> GHMASMAKIKNQYYNESVSPIEYAQQGFKGKMRSVNWNVVNDEKDLEVWNRITQNFWLPEKIPVSNDLTSWRTLTPEWQELITRTFTGLTLLDTIQATVGDVAQVPNSLTDHEQVIYTNFAFMVAVHARSYGSIFSTLCSSEQIEEAHEWVINTETLQERAKALIPYYVNDDP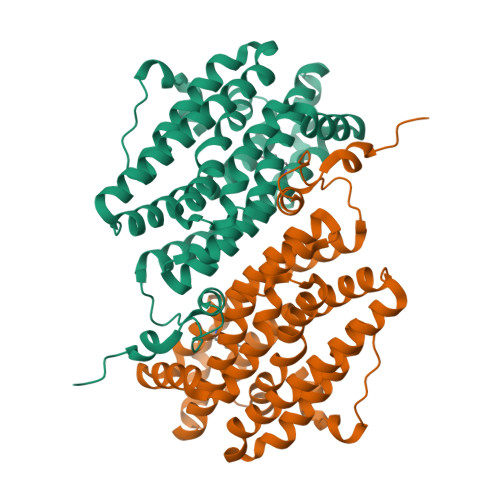LKSKVAAALMPGFLLYGGFYLPFYLSARGKLPNTSDIIRLILRDKVIHNYYSGYKYQKKVAKLSPEKQAEMKEFVFKLLYELIDLEKAYLKELYEDFGLADDAIRFSVYNAGKFLQNLGYDSPFTEEETRIEPEIFTQLSARADENHDFFSGNGSSYIMGVSEETEDDDWEF> LAHSKMVPIPAGVFTMGTDDPQIKQDGEAPARRVTIDAFYMDAYEVSNTEFEKFVNSTGYLTEAEKFGDSFVFEGMLSEQVKTNIQQAVAAAPWWLPVKGANWRHPEGPDSTILHRPDHPVLHVSWNDAVAYCTWAGKRLPT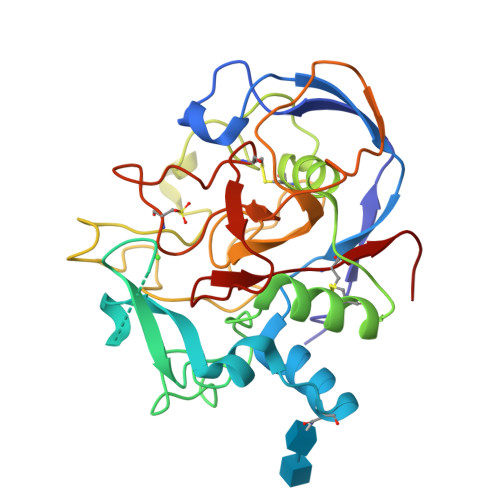EAEWEYSCRGGLHNRLFPWGNKLQPKGQHYANIWQGEFPVTNTGEDGFQGTAPVDAFPPNGYGLYNIVGNAWEWTSDWWTVHHSVEETLNPKGPPSGKDRVKKGGSYMCHRSYSYRYRCAARSQNTPDSSASNLGFRCAADRLP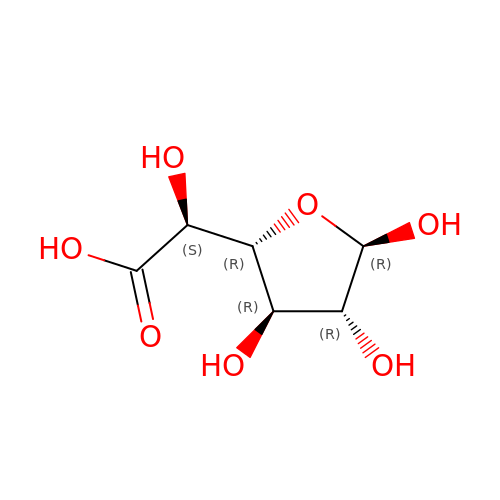beta-D-galactofuranuronic acid | C6 H10 O7 | OEVWLAOZEALENB-ORELYVPDSA-N>MDFKYTEEKETIKINNIMIAKYTVLYTSNCIMDIYSEEEKITCFSNRLVFLERGVNISVRMQKQILSEKPYVAFALNGDMLRHLKDAL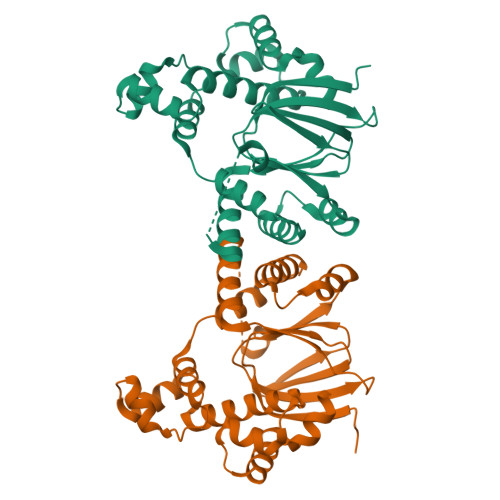MIIYGMSKIDTNACRSMSRKIMTTEVNKTLLDELKNINSHDNSAFISSLIYLISKLENNEKIIESIYISSVSFFSDKVRNLIEKDLSRKWTLGIIADAFNASEITIRKRLESENTNFNQILMQLRMSKAALLLLENSYQISQISNMIGISSASYFIRIFNKHYGVTPKQFFTYFKGG[2x]(4Z,7Z,10Z,13Z,16Z,19R,20R)-19,20-dihydroxydocosa-4,7,10,13,16-pentaenoic 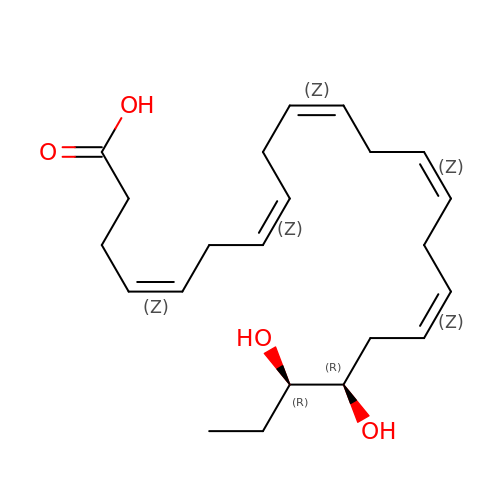acid | C22 H34 O4 | FFXKPSNQCPNORO-KVZKRMIJSA-N The Sec translocon provides the lipid bilayer entry for ribosome‐bound nascent chains and thus facilitates membrane protein biogenesis. The translocon, an integral membrane protein itself, builds a protein‐conducting channel in the lipid bilayer and allows either transmembrane passage of nascent polypeptide chains or their partitioning into the lipid environment as transmembrane α‐helices (TMHs). The central subunit of the translocon, SecY in bacteria or Sec61α in eukaryotes, consists of 10 TMHs arranged as a pseudo‐symmetric “clam‐shell” with a protein‐conducting pore between the N‐ and C‐terminal parts 3, 4. SecY is stabilized at the periphery by the essential subunit SecE/Sec61γ that contains two α‐helices, one in interfacial and one in transmembrane topologies.

Here, we present a cryo‐electron microscopy‐based structure of bacterial translocon SecYEG in lipid nanodiscs and elucidate an early intermediate state upon insertion of the FtsQ anchor domain. Thus, we used an extended scaffold protein MSP1E3D1 and POPG/POPC lipids to reconstitute SecYEG into nanodiscs with a diameter of approximately 12 nm. Thus, to investigate an early stage of the TMH insertion, we prepared translation‐stalled ribosomes, which exposed the first 48 amino acids of FtsQ, including the TMH within the nascent chain (Fig EV1), and incubated those with a 10‐fold excess of SecYEG‐ND to achieve complex formation. After sorting and refinement steps (Fig EV2), the ribosome structure was resolved at 3.3 Å, and independent refinement of the SecYEG‐ND:RNC complex elements led to 3.2 and 3.1 Å resolution for the small (30S) and large (50S) ribosomal subunits, respectively, and was limited to 6 Å for the lipid‐embedded SecYEG due to its small size and apparent dynamics relative to the 50S ribosomal subunit (Movie EV1). In spite of the loose binding of SecYEG to the RNC and its higher flexibility, the complete architecture of essential SecY and SecE subunits was resolved, and a single‐helix density proximate to the SecY N‐terminal domain was assigned to TMH 2 of the SecG subunit, while TMH 1 could not be reliably detected. However, our structure revealed a very different organization of the complex, as SecE TMHs formed a helical hairpin in close proximity to SecY C‐terminal domain, and the hairpin was tilted within the lipid bilayer by ~30°. Surprisingly, the periplasmic loop of the SecE helical hairpin reached TMH 8 and a short helix connecting TMHs 7 and 8 of SecY, and so appeared in direct contact with the lateral gate of the translocon, thus suggesting a potential role of SecE in the translocon gating mechanism but also explaining interactions of SecE with nascent TMHs soon after their membrane partitioning.

> MAKQPGLDFQSAKGGLGELKRRLLFVIGALIVFRIGSFIPIPGIDAAVLAKLLEQQRGTIIEMFNMFSGGALSRASIFALGIMPYISASIIIQLLTVVHPTLAEIKKEGESGRRKISQYTRYGTLVLAIFQSIGIATGLPNMPGMQGLVINPGFAFYFTAVVSLVTGTMFLMWLGEQITERGIGNGISIIIFAGIVAGLPPAIAHTIEQARQGDLHFLVLLLVAVLVFAVTFFVVFVERGQRRIVVNYAKRQQGRRVYAAQSTHLPLKVNMAGVIPAIFASSIILFPATIASWFGGGTGWNWLTTISLYLQPGQPLYVLLYASAIIFFCFFYTALVFNPRETADNLKKSGAFVPGIRPGEQTAKYIDKVMTRLTLVGALYITFICLIPEFMRDAMKVPFYFGGTSLLIVVVVIMDFMAQVQTLMMSSQYESALKKANLKGYGR>NLYFQHMRHFARTHAIGQIVPGKVTKLVPFGAFVRVEEGIEGLVHISEL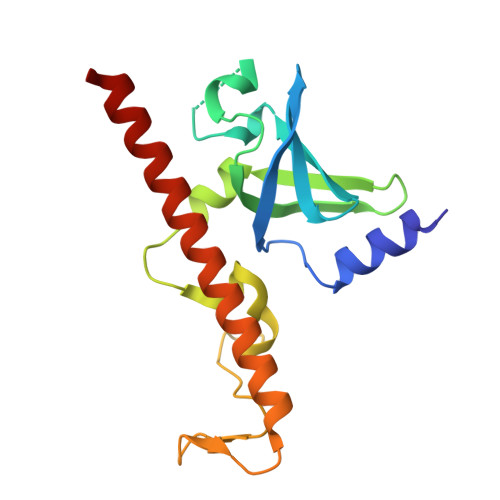SERHVEVPDQVVQVGDDAMVKVIDIDLERRRISLSLKQANEDYTEEFDPSKYGMADSYDEQGNYIFPEGFDPETNEWLEGFDKQREEWEARYAEAERRHKMHTAQMEKFAAAEAEAANA[2x]>[2x]MTPYEDLLRFVLETGTPKSDRTGTGTRSLFGQQMRYDLSAGFPLLTTKKVHFKSVAYELLWFLRGDSNIGWLHEHGVTIWDEWASDTGELGPIYGVQWRSWPAPSGEHIDQIS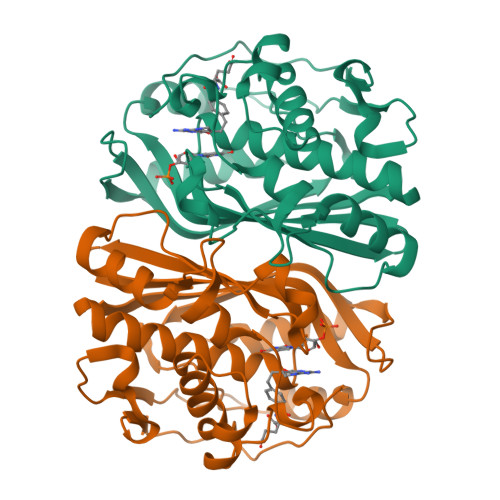AALDLLRTDPDSRRIIVSAWNVGEIERMALPPCHAFFQFYVADGRLSCQLYQRSADLFLGVPFNIASYALLTHMMAAQAGLSVGEFIWTGGDCHIYDNHVEQVRLQLSREPRPYPKLLLADRDSIFEYTYEDIVVKNYDPHPAIKAPVAV>[2x]GPLGSMKIFLENLYHSDCYFLPIRDNQQVLVGVELITHFSSEDGTVRIPTSRVIAQLTEEQHWQLFSEQLELLKSCQHFFIQHKLFAWLNLTPQVATLLLERDNYAGELLKYPFIELLINENYPHLNEGKDNRGLLSLSQVYPLVLGNLGAGNSTMKAVFDGLFTRVMLDKSFIQQQITHRSFEPFIRAIQAQISPCCNCIIAGGIDTAEILAQITPFDFHALQGCLWPAVPINQITTLVQR

The products of flhDC operon, FlhD and FlhC, form a heterohexamer (D4C2) to bind to the upstream of class II promoters and promote class II genes transcription. Recently, two other proteins, FliT and YdiV, are recognized as negative regulators that prevent FlhD4C2 from binding to its target DNA by direct protein–protein interactions. Wada et al. demonstrated that Salmonella YdiV functions as a novel anti-FlhD4C2 factor, which regulates bacterium motility and is responsible for nutritional control of the flagellum regulation in Salmonella. Our structure analyses combined with biochemistry studies and reconstruction of YdiV4–FlhD4C2 structure via negative staining electron microscopy provide a clear regulatory mechanism that stoichiometric binding of YdiV to FlhD in the FlhD4C2 complex results in the opening of the ring-like structure of FlhD4C2 with consequent loss of DNA binding.

The YdiV structure was solved using selenium single-wavelength anomalous diffraction at 1.9 Å resolution. The final model of YdiV contains two protein molecules (Mol A and Mol B) per asymmetric unit. The YdiV monomer consists of 10 α-helices, 8 β-strands and 2 short 310 helices, which exhibits a modified TIM-like barrel fold. Although YdiV shares low-sequence identities with other EAL domain proteins (below 20% for the full length), the topology of the structures is the same. Particularly, the α8-helix of YdiV, which is essential for dimerization in other EAL structures, undergoes dramatic transformation. Notably, although YdiV loses most of the residues coordinating with c-di-GMP, a similar groove that is responsible for c-di-GMP binding in other EAL structures is still retained. Electron density map clearly shows the existence of a phosphate and a glycerol molecule in this groove. The interaction style of YdiV’s Mol A and Mol B is completely different from other dimerized EAL structures, such as Blrp1, YkuI, TBD1265, LapD and FimX. The Mol A and Mol B’s α8-helices, whose corresponding helices mediates the dimerization in Blrp1, YkuI, LapD and TBD1265 structures, are far away from each other. The interaction interface between the two monomers is also smaller than that of the standard EAL protein dimers.>[2x]MACKGTGNRTIAVYDLGGGTFDISIIEIDEVDGEKTFEVLATNGDTHLGG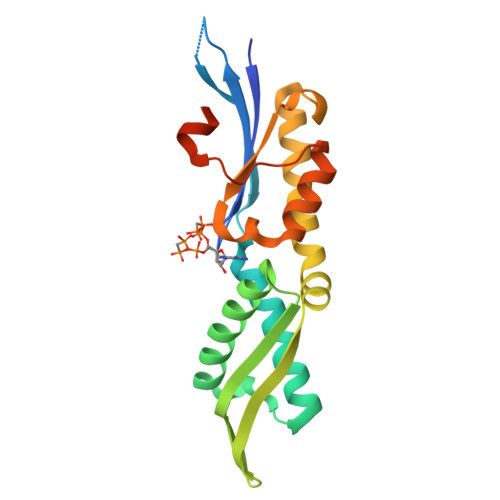EDFDSRLINYLVEEFKKDQGIDLRNDPLAMQRLKEAAEKAKIELSSAQQTDVNLPYITADATGPKHMNIKVTRAKLESLVEDLVNRSIEPLKVALQDAGLSVSDIDDVILVGGQTRMPMVQKKVAEFFGKEPRKDVNPDEAVAIGAAVQGGVLTKCL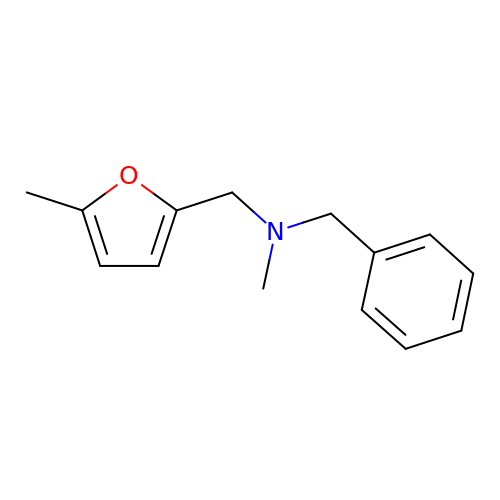~{N}-methyl-~{N}-[(5-methylfuran-2-yl)methyl]-1-phenyl-methanamine | C14 H17 N O | PLXKOSIEYNAHBU-UHFFFAOYSA-N> MGSSHHHHHHSQDPNSHMKETPLSNCERRFLLRAIEEKKRLDGRQTYDYRNIRISFGTDYGCCIVELGKTRVLGQVSCELVSPKLNRATEGILFFNLELSQMAAPAFEPGRQSDLLVKLNRLMERCLRNSKCIDTESLCVVAGEKVWQIRVDLHLLNHDGNIIDAASIAAIVALCHFRRPDVSVQGDEVTLYTPEERDPVPLSIHHMPICVSFAFFQQGTYLLVDPNEREERVMDGLLVIAMNKHREICTIQSSGGIMLLKDQVLRCSKIAGVKVAEITELILKALENDQKVRKEGGKFGFAESIANQRITAFKMEKAPIDTSDVEEKAEEIIAEAEPPSEVVSTPVLWTPGTAQIGEGVENSWGDLEDSEKEDDEGGGDQAIILDGIKMDTGVEVSDIGSQELGFHHVGQTGLEFLTSDAPIILSDSEEEEMIILEPDKNPKKIRTQTTSAKQEKAPSKKPVKRRKKKRAAN;> MADPMAGLELLSDQGYRVDGRRAGELRKIQARMGVFAQADGSAYIEQGNTKALAVVYGPHEIRGSRARALPDRALVNCQYSSATFSTGERKRRPHGDRKSCEMGLQLRQTFEAAILTQLHPRSQIDIYVQVLQADGGTYAACVNAATLAVLDAGIPMRDFVCACSAGFVDGTALADLSHVEEAAGGPQLALALLPASGQIALLEMDARLHEDHLERVLEAAAQAARDVHTLLDRVVRQHVREASILLGD;> DPMAAGFKTVEPLEYYRRFLKENCRPDGRELGEFRTTTVNIGSISTADGSALVKLGNTTVICGVKAEFAAPSTDAPDKGYVVPNVDLPPLCSSRFRSGPPGEEAQVASQFIADVIENSQIIQKEDLCISPGKLVWVLYCDLICLDYDGNILDACTFALLAALKNVQLPEVTI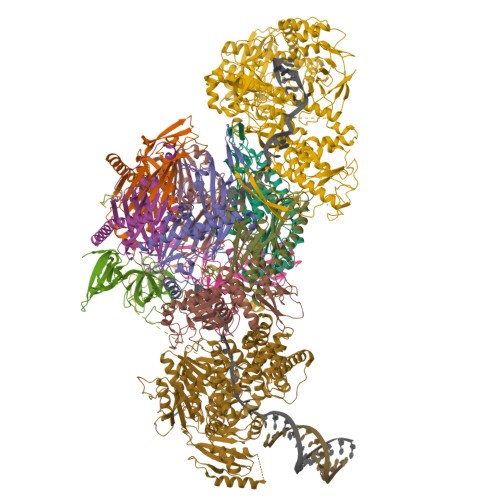NEETALAEVNLKKKSYLNIRTHPVATSFAVFDDTLLIVDPTGEEEHLATGTLTIVMDEEGKLCCLHKPGGSGLTGAKLQDCMSRAVTRHKEVKKLMDEVIKSMKPK;> SLMEEETHTDAKIRAENGTGSSPRGPGCSLRHFACEQNLLSRPDGSASFLQGDTSVLAGVYGPAEVKVSKEIFNKATLEVILRPKIGLPGVAEKSRERLIRNTCEAVVLGTLHPRTSITVVLQVVSDAGSLLACCLNAACMALVDAGVPMRALFCGVACALDSDGTLVLDPTSKQEKEARAVLTFALDSVERKLLMSSTKGLYSDTELQQCLAAAQAASQHVFRFYRESLQRRYSKS;> DPMASVTLSEAEKVYIVHGVQEDLRVDGRGCEDYRCVEVETDVVSNTSGSARVKLGHTDILVGVKAEMGTPKLEKPNEGYLEFFVDCSASATPEFEGRGGDDLGTEIANTLYRIFNNKSSVDLKTLCISPREHCWVLYVDVLLLECGGNLFDAISIAVKAALFNTRIPRVRVLEDEEGSKDIELSDDPYDCIRLSVENVPCIVTLCKIGYRHVVDATLQEEACSLASLLVSVTSKGVVTCMRKVGKGSLDPESIFEMMETGKRVGKVLHASLQSVVHKEESLGPKRQKVGFLG;> MPGDHRRIRGPEESQPPQLYAADEEEAPGTRDPTRLRPVYARAGLLSQAKGSAYLEAGGTKVLCAVSGPRQAEGGERGGGPAGAGGEAPAALRGRLLCDFRRAPFAGRRRRAPPGGCEERELALALQEALEPAVRLGRYPRAQLEVSALLLEDGGSALAAALTAAALALADAGVEMYDLVVGCGLSLAPGPAPTWLLDPTRLEEERAAAGLTVALMPVLNQVAGLLGSGEGGLTESWAEAVRLGLEGCQRLYPVLQQSLVRAARRRGAAAQP;> DPMAEPASVAAESLAGSRARAARTVLGQVVLPGEELLLPEQEDAEGPGGAVERPLSLNARACSRVRVVCGPGLRRCGDRLLVTKCGRLRHKEPGSGSGGGVYWVDSQQKRYVPVKGDHVIGIVTAKSGDIFKVDVGGSEPASLSYLSFEGATKRNRPNVQVGDLIYGQFVVANKDMEPEMVCIDSCGRANGMGVIGQDGLLFKVTLGLIRKLLAPDCEIIQEVGKLHPLEIVFGMNGRIWVKAKTIQQTLILANILEACEHMTSDQRKQIFSRLAES;> DPHMAMEMRLPVARKPLSERLGRDTKKHLVVPGDTITTDTGFMRGHGTYMGEEKLIASVAGSVERVNKLICVKALKTRYIGEVGDIVVGRITEVQQKRWKVETNSRLDSVLLLSSMNLPGGELRRRSAEDELAMRGFLQEGDLISAEVQAVFSDGAVSLHTRSLKYGKLGQGVLVQVSPSLVKRQKTHFHDLPCGASVILGNNGFIWIYPTPEHKEEEAGGFIANLEPVSLADREVISRLRNCIISLVTQRMMLYDTSILYCYEASLPHQIKDILKPEIMEEIVMETRQRLLEQEG;> DPMAPPVRYCIPGERLCNLEEGSPGSGTYTRHGYIFSSLAGCLMKSSENGALPVVSVVRETESQLLPDVGAIVTCKVSSINSRFAKVHILYVGSMPLKNSFRGTIRKEDVRATEKDKVEIYKSFRPGDIVLAKVISLGDAQSNYLLTTAENELGVVVAHSESGIQMVPISWCEMQCPKTHTKEFRKVARVQPEFLQT;> SMAPPSTREPRVLSATSATKSDGEMVLPGFPDADSFVKFALGSVVAVTKASGGLPQFGDEYDFYRSFPGFQAFCETQGDRLLQCMSRVMQYHGCRSNIKDRSKVTELEDKFDLLVDANDVILERVGILLDEASGVNKNQQPVLPAGLQVPKTVVSSWNRKAAEYGKKAKSETFRLLHAKNIIRPQLKFREKIDNSNTPFLPKIFIKPNAQKPLPQALSKERRERPQDRPEDLDVPPALADFIHQQRTQQVEQDMFAHPYQYELNHFTPADAVLQKPQPQLYRPIEETPCHFISSLDELVELNEKLLNCQEFAVNLEHHSYRSFLGLTCLMQISTRTEDFIIDTLELRSDMYILNESLTDPAIVKVFHGADSDIEWLQKDFGLYVVNMFDTHQAARLLNLGRHSLDHLLKLYCNVDSNKQYQLADWRIRPLPEEMLSYARDDTHYLLYIYDKMRLEMWERGNGQPVQLQVVWQRSRDICLKKFIKPIFTDESYLELYRKQKKHLNTQQLTAFQLLFAWRDKTARREDESYGYVLPNHMMLKIAEELPKEPQGIIACCNPVPPLVRQQINEMHLLIQQAREMPLLKSEVAAGVKKSGPLPSAERLENVLFGPHDCSHAPPDGYPIIPTSGSVPVQKQASLFPDEKEDNLLGSRGSGSGSGSGSVSQAAKFDPSTKIYEISNRWKLAQVQVQKDSKEAVKKKAAEQTAAREQAKEACKAAAEQAISVRQQVVLENAAKKRERATSDPRTTEQKQEKKRLKISKK;> GSMLKSKTFLKKTRAGGVMKIVREHYLRDDIGCGAPGCAACGGAHEGPALEPQPQDPASSVCPQPHYLLPDTNVLLHQIDVLEDPAIRNVIVLQTVLQEVRNRSAPVYKRIRDVTNNQEKHFYTFTNEHHRETYVEQEQGENANDRNNRAIRVAAKWYNEHLKKMSADNQLQVIFITNDRRNKEKAIEEGIPAFTCEEYVKSLTANPELIDRLACLSEEGNEIESGKIIFSEHLPLSKLQQGIKSGTYLQGTFRASRENYLEATVWIHGDSEENKEIILQGLKHLNRAVHEDIVAVELLPKSQWVAPSSVVLHDEGQNEEDVEKEEETERMLKTAVSEKMLKPTGRVVGIIKRNWRPYCGMLSKSDIKESRRHLFTPADKRIPRIRIETRQASTLEGRRIIVAIDGWPRNSRYPNGHFVRNLGDVGEKETETEVLLLEHDVPHQPFSQAVLSFLPKMPWSITEKDMKNREDLRHLCICSVDPPGCTDINDALHCRELENGNLEVGVHIADVSHFIRPGNALDQESARRGTTVYLCEKRIDMVPELLSSNLCSLKCDVDRLAFSCIWEMNHNAEILKTKFTKSVINSKASLTYAEAQLRIDSANMNDDITTSLRGLNKLAKILKKRRIEKGALTLSSPEVRFHMDSETHDPIDLQTKELRETNSMVEEFMLLANISVAKKIHEEFSEHALLRKHPAPPPSNYEILVKAARSRNLEIKTDTAKSLAESLDQAESPTFPYLNTLLRILATRCMMQAVYFCSGMDNDFHHYGLASPIYTHFTSPIRRYADVIVHRLLAVAIGADCTYPELTDKHKLADICKNLNFRHKMAQYAQRASVAFHTQLFFKSNGIVSEEAYILFVRKNAIVVLIPKYGLEGTVFFEEKDKPNPQLIYDDEIPSLKIEDTVFHVFDKVKVKIMLDSSNLQHQKIRMSLVEPQIPGISIPTDTSNMDLNGPKKKKMKLGK;> DPMAAERKTRLSKNLLRMKFMQRGLDSETKKQLEEEEKKIISEEHWYLDLPELKEKESFIIEEQSFLLCEDLLYGRMSFRGFNPEVEKLMLQMNAKHKAEEVEDETVELDVSDEEMARRYETLVGTIGKKFARKRDHANYEEDENGDITPIKAKKMFLKPQD;> SGDMADAFGDELFSVFEGDSTTAAGTKKDKEKDKGKWKGPPGSADKAGKRFDGKLQSESTNNGKNKRDVDFEGTDEPIFGKKPRIEESITEDLSLADLMPRVKVQSVETVEGCTHEVALPAEEDYLPLKPRVGKAAKEYPFILDAFQREAIQCVDNNQSVLVSAHTSAGKTVCAEYAIALALREKQRVIFTSPIKALSNQKYREMYEEFQDVGLMTGDVTINPTASCLVMTTEILRSMLYRGSEVMREVAWVIFDEIHYMRDSERGVVWEETIILLPDNVHYVFLSATIPNARQFAEWICHLHKQPCHVIYTDYRPTPLQHYIFPAGGDGLHLVVDENGDFREDNFNTAMQVLRDAGDLAKGDQKGRKGGTKGPSNVFKIVKMIMERNFQPVIIFSFSKKDCEAYALQMTKLDFNTDEEKKMVEEVFSNAIDCLSDEDKKLPQVEHVLPLLKRGIGIHHGGLLPILKETIEILFSEGLIKALFATETFAMGINMPARTVLFTNARKFDGKDFRWISSGEYIQMSGRAGRRGMDDRGIVILMVDEKMSPTIGKQLLKGSADPLNSAFHLTYNMVLNLLRVEEINPEYMLEKSFYQFQHYRAIPGVVEKVKNSEEQYNKIVIPNEESVVIYYKIRQQLAKLGKEIEEYIHKPKYCLPFLQPGRLVKVKNEGDDFGWGVVVNFSKKSNVKPNSGELDPLYVVEVLLRCSKESLKNSATEAAKPAKPDEKGEMQVVPVLVHLLSAISSVRLYIPKDLRPVDNRQSVLKSIQEVQKRFPDGIPLLDPIDDMGIQDQGLKKVIQKVEAFEHRMYSHPLHNDPNLETVYTLCEKKAQIAIDIKSAKRELKKARTVLQMDELKCRKRVLRRLGFATSSDVIEMKGRVACEISSADELLLTEMMFNGLFNDLSAEQATALLSCFVFQENSSEMPKLTEQLAGPLRQMQECAKRIAKVSAEAKLEIDEETYLSSFKPHLMDVVYTWATGATFAHICKMTDVFEGSIIRCMRRLEELLRQMCQAAKAIGNTELENKFAEGITKIKRDIVFAASLYL> GPLGSAFQKCPICEKVIQGAGKLPRHIRTHTGEKPYECNICKVRFTRQDKLKVHMRKHTGEKPYLCQQCGAAFAHNYDLKNHMRVHTGLRPYQCDS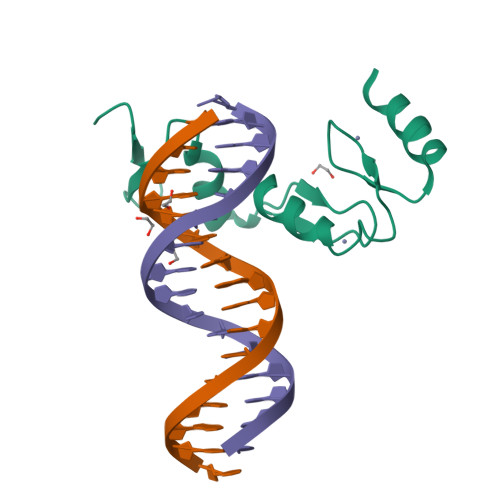CCKTFVRSDHLHRHLKKDGCNGVPSRRGRKLERPHRD>MSLDIEQQFLNDLDNQLWRAADKLRSNLDAANYKHVVLGLIFLKYVSDAFEERQQELTELFQKDDDDNIYYLPREDYDSDEAYQQAIAEELEIGDYYTEKNVFWVPKTARWNKLRDVITLPTGSVIWQDEQGEDVKLRSVSWLIDNAFDDIEKANPKLKGILNRISQYQLDADKLIGLINEFSLTSFNNPEYNGEKLNLKSKDILGHVYEYFLGQFALAEGKQGGQYYTPKSIVTLIVEMLEPYKGRV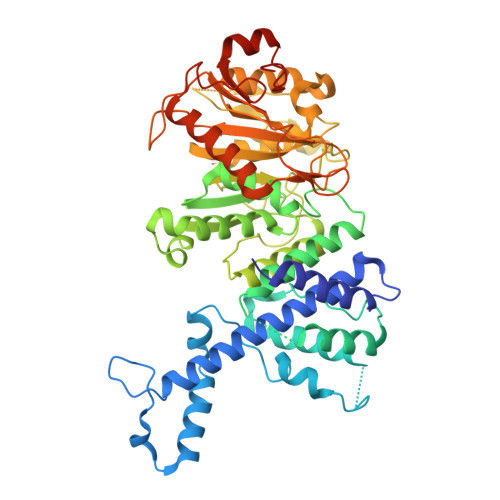YDPAMGSGGFFVSSDKFIEKHANVKHYNASEQKKQISVYGQESNPTTWKLAAMNMVIRGIDFNFGKKNADSFLDDQHPDLRADFVMTNPPFNMKDWWHEKLADDPRWTINTNGEKRILTPPTGNANFAWMLHMLYHLAPTGSMALLLANGSMSSNTNNEGEIRKTLVEQDLVECMVALPGQLFTNTQIPACIWFLTKDKNAKNGKRDRRGQVLFIDARKLGYMKDRVLRDFKDEDIQKLADTFHNWQQEWSEENNQAGFCFSADLALIRKNDFVLTPGRYVGAEAEEDEGHHHHHH[2x]>GPGSMKVISSIQELRDQLRGQNRTAFVPTMGNLHEGHLSLMRLARQHGDPVVASIFVNRLQFGPNEDFDKYPRTLQEDIEKLQKENVYVLFAPTERDMYPEPQEYRVQPPHDLGDILEGEFRPGFFTGVCTVVTKLMACVQPRVAVFGKKDYQQLMIVRRMCQQLALPVEIVAAETVRD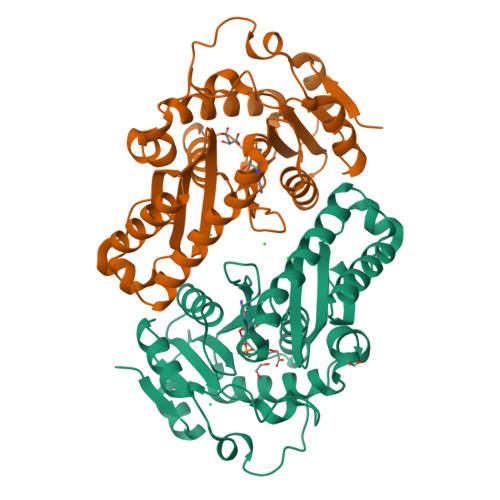ADGLALSSRNRYLSEAERAEAPELAKTLARVRDAVLDGERDLAAIERRAVAHLSARGWQPDYVSIRRRENLVAPSAAQIEAGDPLVVLTAAKLGATRLIDNLEI[2x]One example is rice Pik-1 that comprises an integrated heavy metal-associated (HMA) domain. In the K-type pair, Pik-1 acts as a sensor that binds the AVR-Pik effector via the Pik-1-integrated HMA domain, whereas Pik-2 is required for activation of immune response upon effector recognition (Maqbool et al., 2015; Zdrzałek et al., 2020). RGA5 and Pik-1 detect three unrelated effectors from the rice blast fungus, Magnaporthe oryzae, AVR-Pia/AVR1-CO39 and AVR-Pik, respectively, via their integrated heavy metal-associated (HMA) domains. Functional characterisation of a resurrected ancestral HMA (ancHMA), dating back to early Oryza evolution, revealed that different allelic variants of Pik-1, Pikp-1 and Pikm-1, convergently evolved from the weakly binding ancestral state towards high-affinity binding and recognition of the AVR-PikD effector through different biochemical paths.

To interpret this model from a structural perspective, we attempted to determine crystal structures of the ancHMA domains in complexes with AVR-PikD. Crystallisation screens of the heterologously expressed proteins resulted in crystals of the ancHMALVKIE–AVR-PikD complex, which diffracted to 1.32 Å resolution. The structure revealed an overall architecture of the complex similar to that of previously published co-structures of Pik-HMAs and AVR-PikD (De la Concepcion et al., 2018; De la Concepcion et al., 2021; Maqbool et al., 2015). We note that the MKANK/EMVKE and IAQVV/LVKIE regions map to two of the three interaction interfaces previously described to underpin binding of AVR-PikD, and other AVR-Pik variants, to Pik-HMAs. Among tested constructs, only the Pikp-1:ancHMALVKIE chimera associated with the effector at levels similar to Pikp-1. This indicates that the polymorphic residues in the IAQVV/LVKIE region are critical for the evolution of enhanced AVR-PikD binding in Pikp-1. AncHMALVKIE formed the strongest interaction with AVR-PikD at levels similar to Pikp-HMA, followed by ancHMALAKIE, then ancHMALAQVV, ancHMALAKIV, and ancHMA, which showed weaker interactions; we did not record any significant binding for ancHMALAKVV. These results indicate that the two most recent mutations, Ala-222-Val and Val-230-Glu, collectively referred to as AV-VE, determined HMA transition towards high-affinity AVR-PikD binding. Close inspection of these structures revealed that the Val-230-Glu (V230E) substitution enhances the interaction with AVR-PikD through hydrogen bond formation with His-46. This bond is formed by Glu-230 (E-230) of ancHMALVKIE but absent in Pikm-HMA and ancHMA, which carry Val-230 (V-230) at the structurally equivalent position. We concluded that this shift is consistent with different stoichiometries of the ancHMA–AVR-PikD complexes; while ancHMALVKIE–AVR-PikD formed a two-to-one complex, the constructs with the extension interacted with the effector at a one-to-one ratio.

>[2x]GPGMKQKIVIKVPMASDKCRSKAMALVASTGGVDSVALVGDLRDKIEVVGDGIDSIKLVSALRKKVGHAELLQVS;> GPETGNKYIEKRAIDLSRERDPNFFDHPGIPVPECFWFMFKNNVRQDAGTCYSSWKMDMKVGPNWVHIKSDDNCNLSGDFPPGWIVLGKKRPGF> QNGYENPT;> GSHMSRPPSREIDYTAYPWFAGNMERQQTDNLLKSHASGTYLIRERPAEAERFAISIKFNDEVKHIKVVEKDNWIHITEAKKFDSLLELVEYYQCHSLKESFKQLDTTLKYPYKSRE

Here, we report that Vav2, a guanine nucleotide exchange factor (GEF) for Rho family GTPase, is a novel interaction partner of APP. Through its SH2 domain, Vav2 can bind to the tyrosine-phosphorylated cytoplasmic domains of several membrane receptors and then mediate different extracellular signals to intracellular responses. Increasing evidence has shown that the tyrosine phosphorylation site Y682 in the intracellular tail of APP is crucial for APP function. Our research demonstrated that Vav2 can interact with APP through its SH2 domain which binds directly to the Y682-phosphorylated APP intracellular tail.

A crystal structure of Vav2-SH2 domain in complex with the APP-derived phosphopeptide APP-pY682 (QNG-pY-ENPT, residues 679–686 of APP695) was determined at 2.45 Å resolution, which revealed a conserved recognition mechanism. ITC reported a binding Kd of 0.86 μM for Vav2-SH2 in complex with APP-pY682 peptide and no binding of Vav2-SH2 and APP-Y682. The peptide lies in an extended backbone conformation roughly perpendicular to the central β-strands of the SH2 domain. Phosphotyrosine pY682′ inserts into the canonical pY-binding pocket formed by R680, R698, R700, H719 and K721. The phosphate moiety of pY682′ forms a hydrogen bond network with the side chains of R680, R698 and R700. Residue E683′ (pY + 1) makes hydrophobic interactions with the side chains of residues K718, I720, F756 and L759. Residue P685′ (pY + 3) patches on the surface of the pY + 3 pocket formed by EF and BG loops and makes contacts with T732, S755 and F756. Residue N684′ (pY + 2) does not interact with SH2 domain. However, when bound to Grb2-SH2 domain the peptide adopts a U-shape conformation. This is due to the presence of a bulky Tryptophan residue (W121) in the EF loop of Grb2-SH2, which is a Threonine residue (T732) at the corresponding position of Vav2-SH2. ITC experiments showed that mutation of R680 to Ala in Vav2-SH2 domain nearly abolished its binding with APP-pY682.> MLGPKRCSMVLDVAFVLEGSDKIGEADFNRSKEFMEEVIQRMDVGQDSIHVTVLQYSYMVTVEYPFSEAQSKGDILQRVREIRYQGGNRTNTGLALRYLSDHSFLVSQGAREQAPALVYMVTGNPASDEIK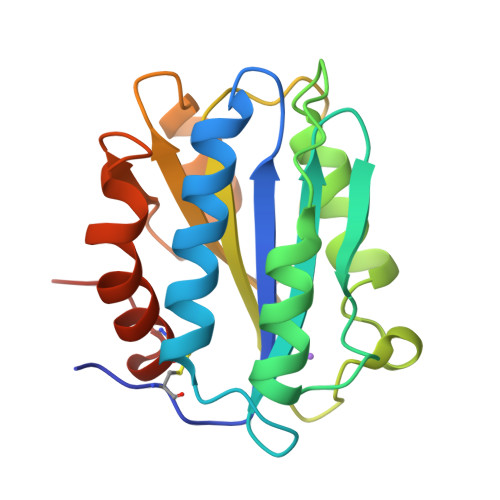RLPGDIQVVPIGVGPNANVQELERIGWPNAPILIQDFETLPREAPDLVLQRCSSGEGLEHHHHHH> MEQNPQSQLKLLVTRGKEQGYLTYAEVNDHLPEDIVDSDQIEDIIQMINDMGIQVMEEAPDADDLMLAENTADEDAAEAAAQVLSSVESEIGRTTDPVRMYMREMGTVELLTREGEIDIAKRIEDGINQVQCSVAEYPEAITYLLEQYDRVEAEEARLSDLITGFVDPNAEEDLAPTATHVGSELSQEDLDDDEDEDEEDGDDDSADDDNSIDPELAREKFAELRAQYVVTRDTIKAKGRSHATAQEEILKLSEVFKQFRLVPKQFDYLVNSMRVMMDR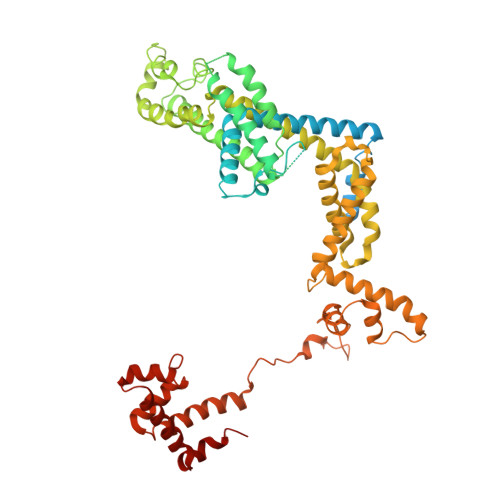VRTQERLIMKLCVEQCKMPKKNFITLFTGNETSDTWFNAAIAMNKPWSEKLHDVSEEVHRALQKLQQIEEETGLTIEQVKDINRRMSIGEAKARRAKKEMVEANLRLVISIAKKYTNRGLQFLDLIQEGNIGLMKAVDKFEYRRGYKFSTYATWWIRQAITRSIADQARTIRIPVHMIETINKLNRISRQMLQEMGREPTPEELAERMLMPEDKIRKVLKIAKEPISMETPIGDDEDSHLGDFIEDTTLELPLDSATTESLRAATHDVLAGLTAREAKVLRMRFGIDMNTDYTLEEVGKQFDVTRERIRQIEAKALRKLRHPSRSEVLRSFLDD>HMLDEPPEGFPEPLNPTNFKEELSKGLHIIDFYSPYCPHCKHLAPVWMETWEEFKEESKTLNITFSQVNCIESADLCGDENIEYFPEIRLYNPSGYIKSFTETPRTKESLIAFARRESMDPNNLDTDLDSAKSESQYLEGFDFLELIAGKATRPHLVSFWPTKDMKNSDDSLEFKNCDKCHEFQRTWKIISRQLAVDDINTGHVNCESNPTICEELGFGDLVKITNHRADREPKVALVLPNKTSNNLFDYPNGYSAKSDGYVDFARRTFTNS[4x]

One of the yeast PDI family members is Eps1p. Based on amino acid sequence, Eps1p appears to be a four-domain protein with a carboxy-terminal membrane anchor. It contains two Cys-X-X-Cys motifs, one in each of the first two Trx domains. The second Eps1p Cys-X-X-Cys motif was also found to be extremely resistant to reduction relative to other PDI family Cys-X-X-Cys motifs.

The refined ND-Eps1p structure was used in turn to solve the structure of S. cerevisiae Esp1p Trx1-Trx2 (SC-Eps1p), crystals of which contained four molecules in the asymmetric unit and diffracted to 2.37 Å resolution. Indeed, the SC-Eps1p structure revealed a different orientation between domains and a different interdomain interface. The interface in SC-Eps1p appears to consist primarily of salt bridges, between helix α4 of the Trx1 domain and helices α2 and α4 of the Trx2 domain, burying about 990 Å2. The distance between the two Cys-X-X-Cys motifs is about 46 Å in the SC-Eps1p structure. The relative domain orientation is the same in all four copies of SC-Eps1p in the asymmetric unit. Another observation regarding the Eps1p Trx2 domain is that the dihedral angles of its Cys-X-X-Cys are relatively uniform in the four molecules in the asymmetric unit of the SC-Eps1p crystals. In contrast, the SC-Eps1p Trx1 Cys-X-X-Cys dihedral angles show greater deviations among the multiple copies of the protein structure. This observation is consistent with the burial of the Trx2 Cys-X-X-Cys motif and its lower temperature factors in all four molecules. In addition, the proline juxtaposed to the Cys-X-X-Cys motif is found in the trans, not cis, configuration in the crystal structures of both Eps1p orthologs.> TDAIAAAT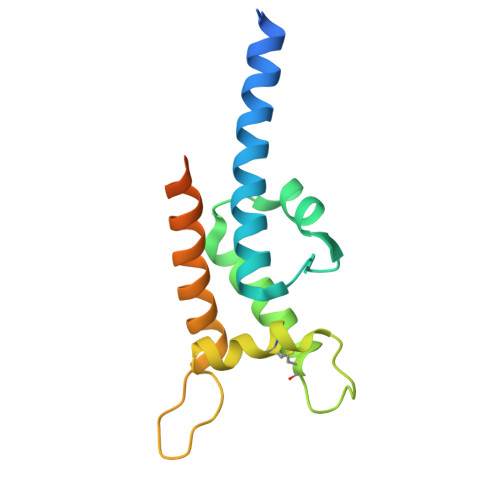KAAMIEGAAQGAVAGEAAGRNAIIGALKRYFHIDNLNGTSLKSFFNSTSYSDVTTIASAIDTQMTASCDAFSGKIVNQAFCDVRKTLRIVADPGKSFVKQKDAITGAVTQLVEKAKDTASFKATEVSSATSSKIITKQNALIE4-propan-2-ylsulfanyl-1-propyl-6,7-dihydro-5~{H}-cyclopenta[d]pyrimidin-2-one 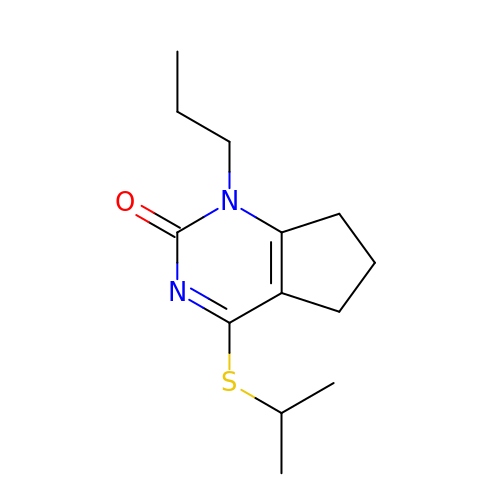| C13 H20 N2 O S | KUWKRQXLULNLGL-UHFFFAOYSA-N Here we investigated the aminopeptidase, P. aeruginosa aminopeptidase (PaAP) from P. aeruginosa, which is highly abundant in the biofilm matrix. PaAP is associated with biofilm development and contributes to nutrient recycling. We confirmed that post-translational processing was required for activation and PaAP is a promiscuous aminopeptidase acting on unstructured regions of peptides and proteins. PaAP contains an M28 Zn peptidase domain (residues 44–116 and 274–510) and a PA domain (residues 117–273).

As a result, we truncated the C-terminus (residues 513–531) by incorporating a C-terminal thrombin cleavage site. This allowed the selective and efficient removal of the C-terminus during purification to produce PaAP_T (a C-terminal truncated form of PaAP). We solved the structure of the truncated enzyme form lacking the final C-terminal residues, PaAP_T, to 2.35 Å, which revealed a large conformational change. Superimposition of the peptidase domains of full-length PaAP and PaAP_T demonstrates the different orientations adopted by the PA domain due to the removal of the C-terminus. The PA domain undergoes an ~40° rotational transition in comparison to the full-length PaAP (20 Å translation at its furthest point). The conformational change increases the opening between the PA and peptidase domain, causing the active site to be more accessible. The rotational swing occurs from the base of the two extended β strands that project from the peptidase domain (starting at P161 and E272). Interestingly, the modified C-terminus (thrombin cleavage site, LVPR) is fully traceable in the PaAP_T structure and binds to the PA domain of an adjacent protomer, where the C-terminus interacts directly with R189A. The interaction of the C-terminus with an adjacent PA domain aids crystal packing, the protomers are linked together, akin to a chain. PaAP_T was highly active in comparison to full-length PaAP (an increase of ~100-fold in kcat, while KM remained unchanged), suggesting the C-terminus is involved in suppressing PaAP activity, in agreement with previous studies.

>[2x]SEAQQFTEFWTPGKPNPSICKSPLLVSTPLGLPRCLQASNVVKRLQKLEDIASLNDGNRAAATPGYQASVDYVKQTLQKAGYKVSVQPFPFTAYYPKGPGSLSATVPQPVTYEWEKDFTYLSQTEAGDVTAKVVPVDLSLGAGNTSTSGCEAEDFANFPAGSIALIQRGTCNFEQKAENAAAAGAAGVIIFNQGNTDDRKGLENVTVGESYEGGIPVIFATYDNGVAWSQTPDLQLHLVVDVVRKKTETYNVVAETRRGNPNNVVMVGAHLDSVFEGPGINDNGSGSAAQLEMAVLLAKALPVNKVRFAWWGAEEAGLVGSTHYVQNLAPEEKKKIKAYLNFDMIGSPNFGNFIYDGDGSDFGLQGPPGSAAIERLFEAYFRLRGQQSEGTEIDFRSDYAEFFNSGIAFGGLFTGAEGLKTEEQAQKYGGTAGKAYDECYHSKCDGIANINQDALEIHSDAMAFVTSWLSLSTKVVDDEIAAAGQKLVPR> FTLIELMIVIAIVGILAAVALPAYQDYTARAQVSEAILLAEGQKSAVTEYYLNHGEWPGDNSSAGVATSAD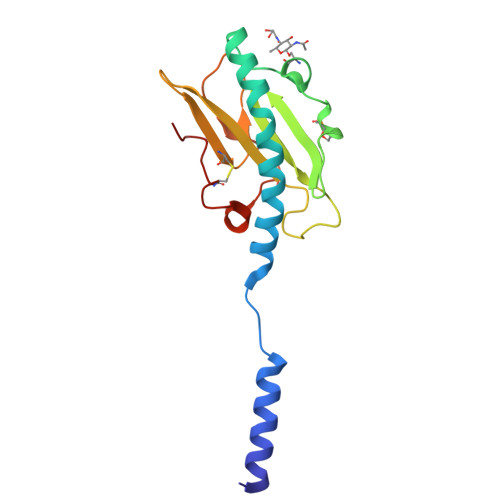IKGKYVQSVTVANGVITAQMASSNVNNEIKSKKLSLWAKRQNGSVKWFCGQPVTRTTATATDVAAANGKTDDKINTKHLPSTCRDDSSAS> MQQLNENKIIKLLRDNIPKLQLIYLFGSYSQGTQHRNSDIDIAVLAADTLDNI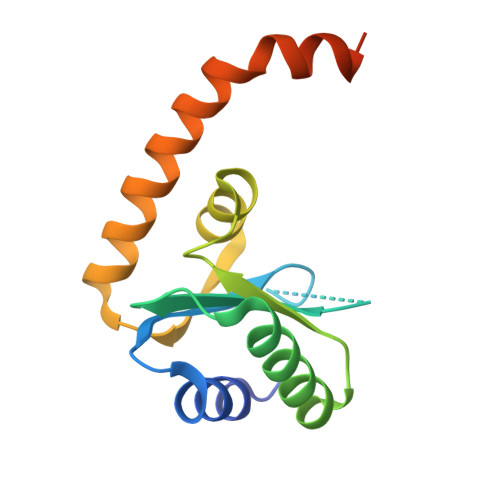ARWELAQKLASALDSDVDLVDLRSASTVLCQQVVTQGKQLWGTQQDDELFAVKTISMYQHLQAERQAIIDDVMANTAAKAHRGESL> MSSGFHFHDVSNDAIKGMPPSEALHKHLENAQLAHRICLAKALKAGEPPVEKCALTWGEVLIRYQAWSEYRPPFQDSVAQAKYKKYWSKKRQEEDDK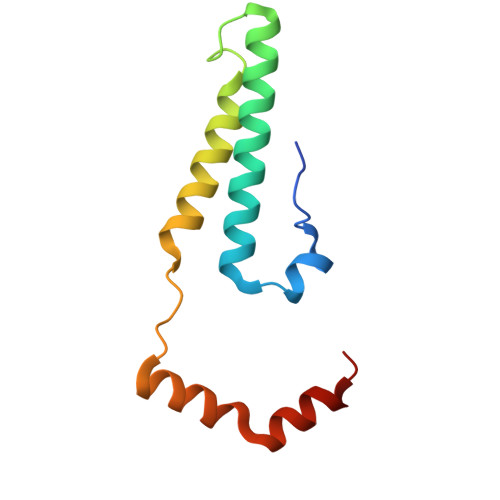NPFK> MDETGKFLVLALYDYQEKSPREVTMKKGDILTLLNSTNKDWWKVEVNGRQGFV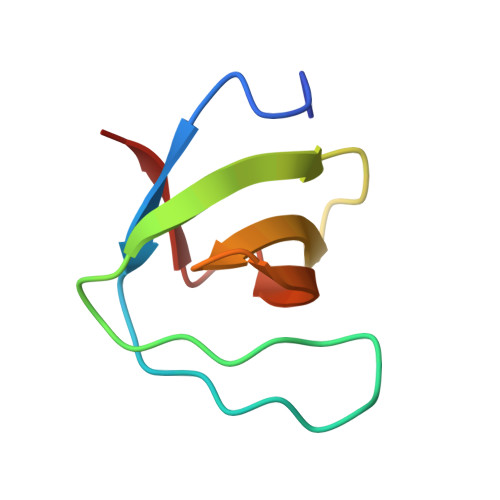PAAYVKFLD> MSLKDVSLSSFDAHDLDLDKFPEVVRDRLTQFLDAQELTIADIGAPVTDAVAHLRSFVLNGGKRIRPLYAWAGFLAAQGHKNSSEKLESVLDAAASLEFIQACALIHDDIIDSSDTRRGAPTVHRAVEADHRANNFEGDPEHFGVSVSILAGDMALVWAEDMLQDSGLSAEALARTRDAWRGMRTEVIGGQLLDI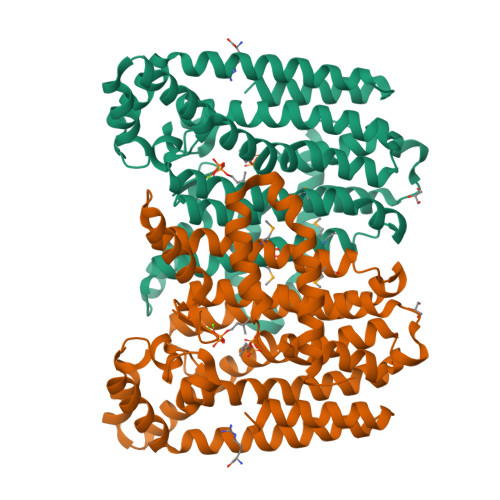YLESHANESVELADSVNRFKTAAYTIARPLHLGASIAGGSPQLIDALLHYGHDIGIAFQLRDDLLGVFGDPAITGKPAGDDIREGKRTVLLALALQRADKQSPEAATAIRAGVGKVTSPEDIAVITEHIRATGAEEEVEQRISQLTESGLAHLDDVDIPDEVRAQLRALAIRSTERREGHHHHHH>[6x]PIVDTGSVAPLSAAEKTK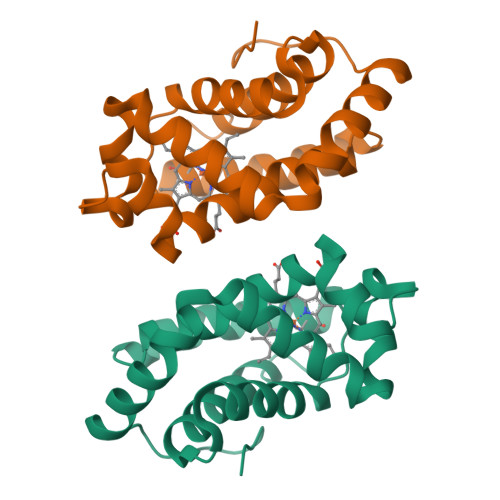IRSAWAPVYSTYETSGVDILVKFFTSTPAAQEFFPKFKGLTTADQLKKSADVRWHAERIINAVNDAVASMDDTEKMSMKLRDLSGKHAKSFQVDPQYFKVLAAVIADTVAAGDAGFEKLMSMICILLRSAY> MLTAQTKNTQTLMPLTERVNVQADSARINQIIDGCWVAVGTNKPHAIQRDFTNLFDGKPSYRFELKTEDNTLEGYAKGETKGRAEFSYCYATSDDFKGLPADVYQKAQITKTVYHHGKGACPQGSSRDYEFSVYIPSSLDSNVSTIFAQWAGMPDRTLVQTPQGEVKKLTVDEFVELEKTTFFKKNAGHEKVVRLDKQGNPMKDKNGKPVYKAGKLNGWLVEQGGYPPLAFGFSGGLFYIKANSDRKWLTDKDDRCNANPGKTPVMKPLTSEYKASTIAYKLPFADFPKDCWITFRVHIDWTVYGKEAETIVKPGMLDVRMDYQEQGKKVSKHIVNNEKILIGRNDEDGYYFKF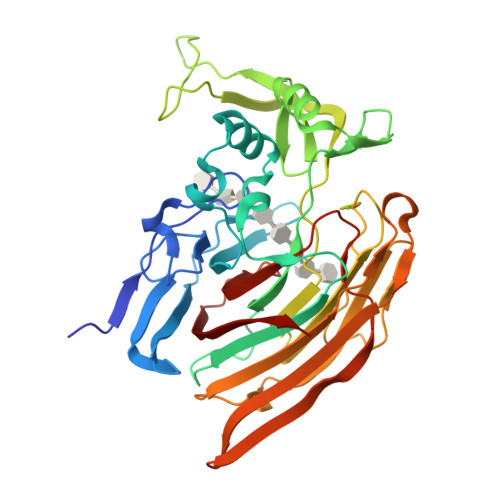GIYRVGDSTVPVCYNLAGYSERLE The folate metabolism enzyme MTHFD2 (methylenetetrahydrofolate dehydrogenase/cyclohydrolase) is consistently overexpressed in cancer but its roles are not fully characterized, and current candidate inhibitors have limited potency for clinical development. Indeed, the one-carbon metabolism enzyme MTHFD2 stands out as the most consistently overexpressed metabolic enzyme across human tumors. MTHFD2 enzymatic function supports rapid cell proliferation during early embryogenesis, after which it is replaced by the mitochondrial protein MTHFD2L in healthy mature tissue.

The tool compound TH7299, as well as two of the most promising candidates, TH9028 and TH9619, were chosen to investigate the MTHFD2 mechanism of action and cancer biology. Furthermore, we determined the cocrystal structures of TH7299, TH9028 and TH9619 in complexes with human MTHFD2 to assess their binding mode and identify critical interactions in the binding pocket. At a predetermined temperature of 57 °C, isothermal dose–response fingerprint (CETSAITDRF) analysis of TH7299, TH9028 and TH9619 in HL-60 cells accurately reflected their relative potencies in biochemical and viability assays, as well as demonstrating the difference in target stabilization potential for TH9619 in nontumorigenic lymphoblastoid cell line (LCL)-889 cells compared with HL-60 AML cells. Treatment with TH7299 resulted in approximately 50% reduction of RF speed and significantly shorter DNA fibers; meanwhile supplementation with thymidine was sufficient to fully rescue replication speeds. To assess the cancer specificity of the replication defects caused by MTHFD2 inhibitors, we treated AML and nontumorigenic LCL cells with TH7299, TH9619, MTX or the ATR inhibitor VE-821. Although MTX and VE-821 significantly blocked DNA RF progression in both cancer and nontumorigenic cells, MTHFD2 inhibitors effectively impaired DNA replication only in AML cells, sparing nontumorigenic lymphocytes. In accordance with this, we found that MTHFD2 inhibitors TH7299 and TH9619 are synergistic when combined with ATR inhibitors VE-821 or VE-822 in both AML HL-60 and THP-1 cells, as well as in bone cancer cell lines U2OS and TC71, increasing apoptosis in a time- and dose-dependent manner.

> MEAVVISGRKLAQQIKQEVRQEVEEWVASGNKRPHLSVILVGENPASHSYVLNKTRAAAVVGINSETIMKPASISEEELLNLINKLNNDDNVDGLLVQLPLPEHIDERRICNAVSPDKDVDGFHVINVGRMCLDQYSMLPATPWGVWEIIKRTGIPTLGKNVVVAGRSKNVGMPIAMLLHTDGAHERPGGDATVTISHRYTPKEQLKKHTILADIVISAAGIPNLITADMIKEGAAVIDVGINRVHDPVTAKPKLVGDVDFEGVRQKAGYITPVPGGVGPMTVAMLMKNTIIAAKKVLRLEEREVLKSKELGVATN> AATTQIGEIVKTVANTVESEIKAELGVIPSLNAVETGATSNTEPEEAIQTRTVINMHGTAECLVENFLGRSALVCMRSFEYKNHSTSTSSIQKNFFIWTLNTRELVQIRRKMELFTYLRFDTEITIVPTLRLFSSSNVSFSGLPNLTLQAMYVPTGARKPSSQDSFEWQSACNPSVFFKINDPPARLTIPFMSINSAYANFYDGFAGFEKKATVLYGINPANTMGNLCLRVVNSYQPVQYTLTVRVYMKPKHIKAWAPRAPRTMPYTNILNNNYAGRSAAPNAPTAIVSHRSTIKTMPNDINLTTA;> SPSAEACGYSDRVLQLKLGNSSIVTQEAANICCAYGEWPTYLPDNEAVAIDKPTQPETSTDRFYTLKSKKWESNSTGWWWKLPDALNQIGMFGQNVQYHYLYRSGFLCHVQCNATKFHQGTLLIVAIPEHQIGKKGTGTSASFAEVMKGAEGGVFEQPYLLDDGTSLACALVYPHQWINLRTNNSATIVLPWMNSAPMDFALRHNNWTLAVIPVCPLAGGTGNTNTYVPITISIAPMCAEYNGLRNAITQ;> GVPTCLLPGSNQFLTTDDHSSAPAFPDFSPTPEMHIPGQVHSMLEIVQIESMMEINNVNDASGVERLRVQISAQSDMDQLLFNIPLDIQLEGPLRNTLLGNISRYYTHWSGSLEMTFMFCGSFMTTGKLIICYTPPGGSSPTDRMQAMLATHVVWDFGLQSSITIIIPWISGSHYRMFNTDAKAINANVGYVTCFMQTNLVAPVGAADQCYIVGMVAAKKDFNLRLMRDSPDIGQSAILPEQ

Enterovirus 70 (EV70) is a human pathogen belonging to the family Picornaviridae. EV70 is transmitted by eye secretions and causes acute hemorrhagic conjunctivitis, a serious eye disease. The capsid of EV70 is composed of the subunits VP1, VP2, VP3, and VP4. The major capsid proteins of EV70 are organized with pseudo-T=3 icosahedral symmetry, with VP1 subunits forming pentamers around 5-fold symmetry axes and VP2 and VP3 subunits forming heterohexamers at 3-fold axes of the capsid.

The structures of altered and empty particles of EV70 were determined to resolutions of 3.7 and 4.3 Å, respectively. The empty particle of EV70 is structurally similar to the altered particle but has the interpentamer binding interface decreased to 1,650 Å2 and the rectangular pores on 2-fold axes of the empty particle expanded to 25 by 16 Å. This pore expansion is caused mostly by the loss of the structure of a helix formed by residues 90 to 98 of VP2. Nevertheless, the residues forming the helix, even though flexible, are still located in the vicinity of the pore. The best-resolved part of the capsid of the empty particle is the intrapentamer interface formed by VP1 subunits, showing that the contacts within a pentamer are more stable than those between pentamers. Although the pore located on a 2-fold axis of the empty particle may enable the exit of a single-stranded RNA, as was proposed previously for EV-D68 (56), we cannot rule out that genome release is enabled by particle opening, as was proposed previously for echoviruses 18 and 30 (43). Because of the low number of images of empty EV70 particles in our data set, we were unable to identify the presence of open particles in the sample.>MTEHPRAHTAHLRTARLELTPLDPAADARHLHHAYGDEEVMRWWTRPACADPAETERYLTSCAAAPGARLWTIRAPDGTVPGMAGLLGGTDVPGLTWLLRRDSWGHGYATEAAAAVVGHALEDGGLDRVEAWIEAGNRRSLAVAARVGLTERARLAQHYPHRPGPHEMVVLGKARAEEPLTTLAVITELPVRDVAATLRLVEAALGARTAFAIGDPPEFAEA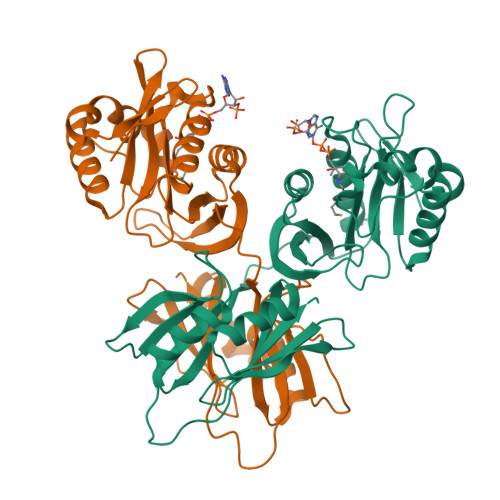ALTPWSAGPRFRLAAVPGPGPVEPVRLHLDAAGTADSLHRRAVDAGARVDGPPVRRPWGRSEFVITLPEGHELTVSAPV[2x]> GSAGTLAAPTAVTSGQSLTSLTAFAYNGTQYQSGGNASINFVATE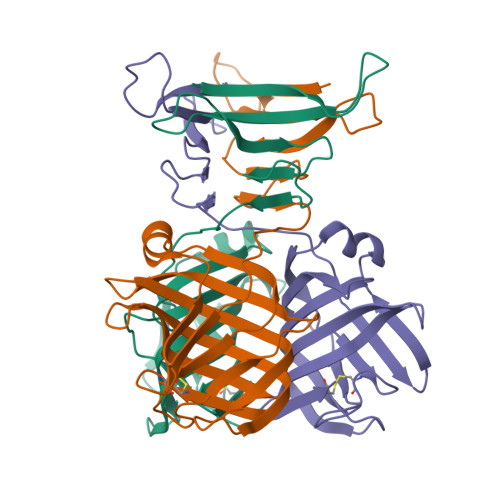AHTASAGGAKIIFNTTNNGATGSTEKVVIDQNGNVGVGVGAPTAKMDVNGGIKQPNYGIISAVRNSGGVTASMPWTNAYVLAHQGEMHQWVAGGPILQDSVTGCNAGPDAGVKFDSIATSWGGPYKVIFHTTGSNGAIHLEWSGWQVSLKNSAGTELAIGMGQVFATLHYDPAVSNWRVEHMFGRINNTNFTCW> MTSLNDIVNKLSSSKIKTRSDALQNLRSYIIYSRNGNSLNQEDALIIEKAIKRAFELEWQISANHGKRQISKASQEQKLQDISYLLRTCVESYILLFREPHILALLDIILRHTFTANGSICEVVCLNFSKALRLLLSHSPHLHHLRFSDWQSLVSYCCQAIEKLSIAEETYVSDSEEEPISQKNYQEISIWKSHDVIRVKQEVVELIYVMRSLVQWYAAPINFVSEQLLKFFEFFFYAYTEETDAHLPALQCLFQLCAYAIPNCNDYSASVVLLVFKILINSDKWKRLDLRLQLIQCLAISYPLWSNSETWDPHRSIRSFNLDLLNSSFFSLKNFLNFFGKRSSLSLANFRFHTVEPKNNIAKLYDPRLHLFFSLRHNSFFESYFIYFFLAKLILLKKTVLSLASTEQANKKQKTCSQIEELLLQAELANISASSFSLQLMVIITAISDNLTNDDLLSIQKMSLNFTEKKNELQSWSFFILFNICYNKAYSSMLTTSCKKEILAAASRGLLNSVTSPVCYQILTYFNMYRPLCFASIFPFIKQQFILFNDYSPMLSYEAIDYWKSLYILLNENLFVGQSSFKSVFLKWLKWHLYHLFSKEGELPFFSFTDSSIIIFDLLMMIFYRPLSLSYITTEIRSPFERNLFHLKEAWSPVTLRFPYTTDEICKQSTEGCYPFNSNHTIDCDSLQNVIKMLESSIDEISSASYDKDELDKETPSFEAVMIFSQISFLCGFLNCFIQKKGIHNVTPNNLVIFKNLFPEVLSFVKSNHSYDPIINCISTNLQFTISDEPKHLRYEIGSDLIRSTHFRDSNPLKTLVLYIMDMASKNVFIKPQEFDHDEYFSQEEEDIYRPENLIRNHQILGLMEGSLEQIRNTDLFILQKYIDYFSSHPHDSLINILHLYPIETFCFGMSAIGAYFLDVARTSEPIFYKCLEILAQKILMNYDYERDEVYLMIFIKIFQKCVHSKLQFTDATLKLIVKITKFIEKVFIETKFSSLSGRQTFLKFIFQLSPTSHVYSKFDYQKLISLTLKDSDVCVIYNFVDDLVIFLKKCDKTLIEGFVLPILSIKIEKSLYKGFCYLYLTLKVFLSISSNRSALLYQLLKLANSYETSTIFEPLLRKLHIQSANIKQLFRIYRLEIFWSFVSKDLSNTTNDFLEFPYKPIYFSLSDFLKENSDEIILVLILTKNITLAKLITSRMSVDFSEKYTQLIPVITTYTHLSEVENKKYSLRFNSIDEALDVELLNRSKAFLFCLEMLKEVKELGSTFKSISSTSFKVYSQLTIFANRVSFNNSTAIPFFSTKSVLWYCNRLFQELEGFSSIPSVIDLVLRRLAIQLHFATDEELQVTISFRLCAFLCFSDPFITSNYLVMIVLRIARQLLSIPCTQSLGLGIARFHLKKFKPTDFDYFFQLAEFCMDFLGFCYNTIGTKMEAIQDFYTWFDGYVTALLNFEYEGYGFLRCQINFVRSVMTTKNEWIEVSNKLFERGHFLKRIAMNNYLCLYFWQVLDACPRNVLHSLSLEIWKCYKAYDITEFPDSLKLFFSDIMGWNFFKSPEIADLNHYIPKTDPRLCDTKTYEESK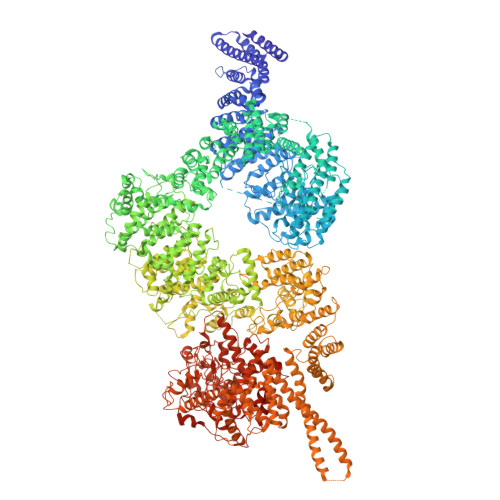LIIWKLICQKACSLLFKYDILLDSFIEDCIRMFFENGNHQELRKFLNFPKDSIIYDSDFKTLVSEEGSFQWVKLQPTNFDSLSNWTKEETLKLLNMMGKSSTTHSLKLLSTYMVGFSTSIIQYIIHLILLEFDFNGNNKKQKEYVTQLILSGLLNKNTNSIRKTCMNILLYLRRQLGHHALNPFEANYWVPINYSVAASTAYDCHLYEQSLLFLTIHNTKTDELDITLLSDILSQLPCPDAYYGIKRETSFKNILLKAVHEKRSPLAISYLDAANMYRSNEDEGTKMMFSNTLNNAGFFSLNEFYIDSLKANDAIDECSNEVYASAWRMQKWDIPPLSLDNKTTKDCLVFEVLHAVHNYAIYGNYLHLEEYINKKLLLINPNEEPDSLLFYALAYDLKFLIRCNQSQFNCDILQLLKENKQMSSQLHECFQLLLEIRNVLLSLLQSHKQLDLSDDLASFRKYYILELLKISESFLIVDNLQNAFSVAMLSDALYRKFDLADENLKHDIDFLSSKILWQRDEKIDAIGMLSESLSKTNSSIFPSISYAYLGNWLYTTKSEKTELVSKNYFEKSLSHMSHLNAKEKAKIYCMFAQFCDNNYSSPDLTEDFKRMEKLYFEKKNDIQQLERSIVNASNMKEEKMLKNHHSREMSSFIIDEREYLRMSTFRSKMLTQSITHYLKCLSESDENDVLISRCCTMWLSNSHLDELNNSLQHYLQNLPCKKFIPVFYQLAARLMNENSKFQQSLTSICYNVGRNHPYHSLHVLFSLVSNVPEIENLDAGSRYRAVKKILDLLKVNQGLSNLVTKLLCSFENYVSLAEWNPRSKVDSTSFSRFPGYKWFLKDAANYGLPPITMNVKVNDTGDYSNIPTVSSFDDTIHFASGINAPKVITCLGSNGHTYKQLVKGGNDDLRQDAVMEQVFEQVNGFLRSYRKTSQRNLSMRTYKVIPLALKTGVIEWVQDTIPLGEYLDSAHKVYHPKEWSLSTCRKLIAEKQMEDLETRLKVYDLVCRHYRPVFRHFFLESYADPVQWFTTQTNYARSTAVASVLGHVLGLGDRHGQNILIDKTSGEVIHIDLGIAFEQGKKLPVPECVPFRLTRDVVDGMGITGVEGVFRRCMEFTLETLRREEDSLLSVLEVLRYDPLFSWLISPLRRMKKQKMQLENFNQPESGNITTDASRDPKIQRNNVSGESEAERAILKVRQKLSSTLSVEASVGELIRIAQDPSYLALMFCGWSAFQ N-{4-[(4S)-2,5-dioxoimidazolidin-4-yl]phenyl}acetamide 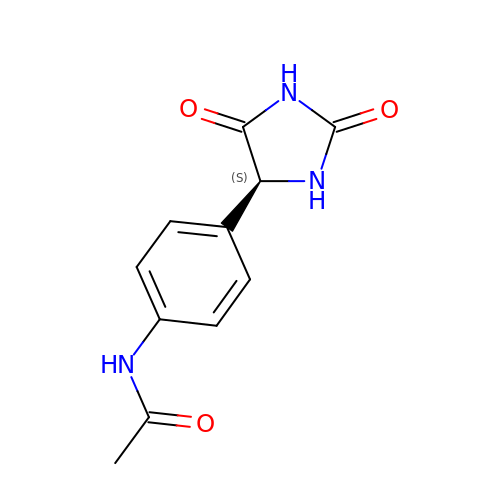| C11 H11 N3 O3 | GUTQNQMNYWTMBT-VIFPVBQESA-N> GPGGSGGVTEEQVHHIVKDALQRYSEDRIGLADYALESGGASVISTRCSETYETKTALISLFGIPLWYHSQSPRVILQPDVHP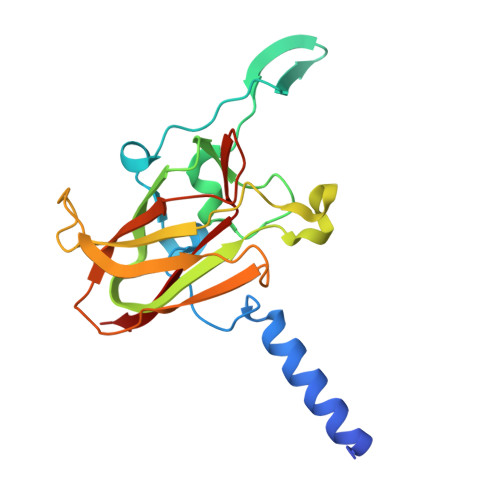GNCWAFQGPQGFAVVRLSARIRPTAVTLEHVPKALSPNSTISSAPKDFAIFGFDEDLQQEGTLLGKFTYDQDGEPIQTFHFQAPGRGTYQVVELRILTNWGHPEYTCIYRFRVHGEPAH> MAHHHHHHDYGIPTTENLYFQGSNPNYCFAGKTSSISDLKEVPRKNITLIRGLGHGAFGEVYEGQVSGMPNDPSPLQVAVKTLPEVCSEQDELDFLMEALIISKLNHQNIVRCIGVSLQSLPRFILLELMAGGDLKSFLRETRPRPSQPSSLAMLDLLHVARDIACGCQYLEENHFIHRDIAARNCLLTCPGPGRVAKIGDFGMARDIYRASYYRKGGCAMLPVKWMPPEAFMEGIFTSKTDT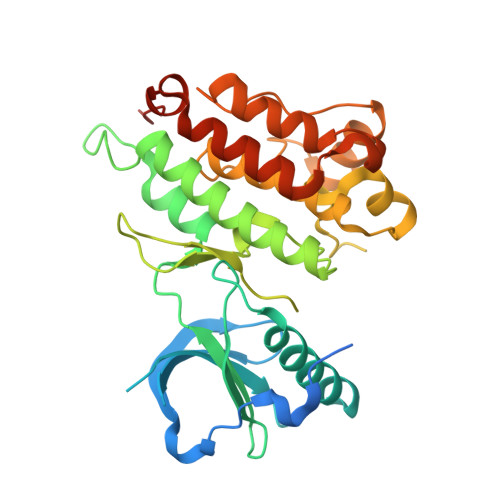WSFGVLLWEIFSLGYMPYPSKSNQEVLEFVTSGGRMDPPKNCPGPVYRIMTQCWQHQPEDRPNFAIILERIEYCTQDPDVINTALPIEYGPLVEEEEKV>[16x]MAAPARDPPGYRYAAAMVPTGSILSTIEVASHRRLFDFFARVRSDENSLYDVEFDALLGSYCNTLSLVRFLELGLSVACVCTKFPELAYMNEGRVQFEVHQPLIARDGPHPVEQPVHNYMTKVIDRRALNAAFSLATEAIALLTGEALDGTGISLHRQLRAIQQLARNVQAVLGAFERGTADQMLHVLLEKAPPLALLLPMQRYLDNGRLATRVARATLVAELKRSFCDTSFFLGKAGHRREAIEAWLVDLTTATQPSVAVPRLTHADTRGRPVDGVLVTTAAIKQRLLQSFLKVEDTEADVPVTYGEMVLNGANLVTALVMGKAVRSLDDVGRHLLDMQEEQLEANRETLDELESAPQTTRVRADLVAIGDRLVFLEALEKRIYAATNVPYPLVGAMDLTFVLPLGLFNPAMERFAAHAGDLVPAPGHPEPRAFPPRQLFFWGKDHQVLRLSMENAVGTVCHPSLMNIDAAVGGVNHDPVEAANPYGAYVAAPAGPGADMQQRFLNAWRQRLAHGRVRWVAECQMTAEQFMQPDNANLALELHPAFDFFAGVADVELPGGEVPPAGPGAIQATWRVVNGNLPLALCPVAFRDARGLELGVGRHAMAPATIAAVRGAFEDRSYPAVFYLLQAAIHGSEHVFCALARLVTQCITSYWNNTRCAAFVNDYSLVSYIVTYLGGDLPEECMAVYRDLVAHVEALAQLVDDFTLPGPELGGQAQAELNHLMRDPALLPPLVWDCDGLMRHAALDRHRDCRIDAGGHEPVYAAACNVATADFNRNDGRLLHNTQARAADAADDRPHRPADWTVHHKIYYYVLVPAFSRGRCCTAGVRFDRVYATLQNMVVPEIAPGEECPSDPVTDPAHPLHPANLVANTVNAMFHNGRVVVDGPAMLTLQVLAHNMAERTTALLCSAAPDAGANTASTANMRIFDGALHAGVLLMAPQHLDHTIQNGEYFYVLPVHALFAGADHVANAPNFPPALRDLARHVPLVPPALGANYFSSIRQPVVQHARESAAGENALTYALMAGYFKMSPVALYHQLKTGLHPGFGFTVVRQDRFVTENVLFSERASEAYFLGQLQVARHETGGGVNFTLTQPRGNVDLGVGYTAVAATATVRNPVTDMGNLPQNFYLGRGAPPLLDNAAAVYLRNAVVAGNRLGPAQPLPVFGCAQVPRRAGMDHGQDAVCEFIATPVATDINYFRRPCNPRGRAAGGVYAGDKEGDVIALMYDHGQSDPARPFAATANPWASQRFSYGDLLYNGAYHLNGASPVLSPCFKFFTAADITAKHRCLERLIVETGSAVSTATAASDVQFKRPPGCRELVEDPCGLFQEAYPITCASDPALLRSARDGEAHARETHFTQYLIYDASPLKGLSL;>[10x]MITDCFEADIAIPSGISRPDAAALQRCEGRVVFLPTIRRQLALADVAHESFVSGGVSPDTLGLLLAYRRRFPAVITRVLPTRIVACPVDLGLTHAGTVNLRNTSPVDLCNGDPVSLVPPVFEGQATDVRLESLDLTLRFPVPLPTPLAREIVARLVARGIRDLNPDPRTPGELPDLNVLYYNGARLSLVADVQQLASVNTELRSLVLNMVYSITEGTTLILTLIPRLLALSAQDGYVNALLQMQSVTREAAQLIHPEAPMLMQDGERRLPLYEALVAWLAHAGQLGDILALAPAVRVCTFDGAAVVQSGDMAPVIRYP;>[5x]MKTKPLPTAPMAWAESAVETTTSPRELAGHAPLRRVLRPPIARRDGPVLLGDRAPRRTASTMWLLGIDPAESSPGTRATRDDTEQAVDKILRGARRAGGLTVPGAPRYHLTRQVTLTDLCQPNAERAGALL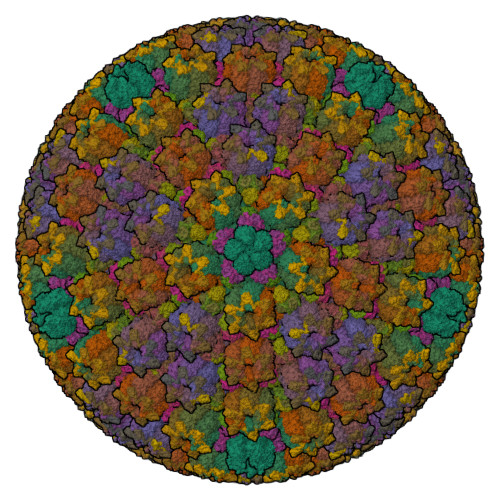LALRHPTDLPHLARHRAPPGRQTERLAEAWGQLLEASALGSGRAESGCARAGLVSFNFLVAACTAAYDARDAAEAVRAHITTNYGGTRAGARLDRFSECLRAMVHTHVFPHEVMRFFGGLVSWVTQDELASVTAVCSGPQEATHTGHPGRPCSAVTIPACAFVDLDAELCLGGPGAAFLYLVFTYRQCRDQELCCVYVVKSQLPPRGLEAALERLFGRLRITNTIHGAEDMTPPPPNRNVDFPLAVLAASSQSPRCSASQVTNPQFVDRLYRWQPDLRGRPTARTCTYAAFAELGVMPDDSPRCLHRTERFGAVGVPVVILEGVVWRPGGWRACA;>MAAPQFHRPSTITADNVRALGMRGLVLATNNAQFIMDNSYPHPHGTQGAVREFLRGQAAALTDLGVTHANNTFAPQPMFAGDAAAEWLRPSFGLKRTYSPFVVRDPKTPSTP[15x]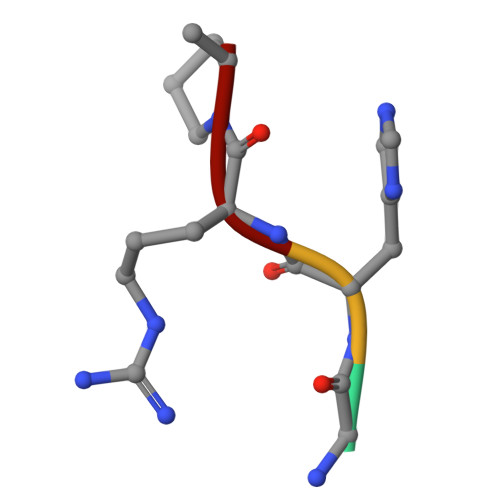> GHRP> GAMASSNTAATNADSAWLEAQEEEEVGFPVRPQVPLRPMTYKAALDISHFLKEKGGLEGLIWSQRRQEILDLWIYHTQGYFPDWQNYTPGPGIRYPLTFGWCFKLVPVEPEKVEEANEGENNSLLHPMSLHGMEDAEKEVLVWRFDSKLAFHHMARELHPEY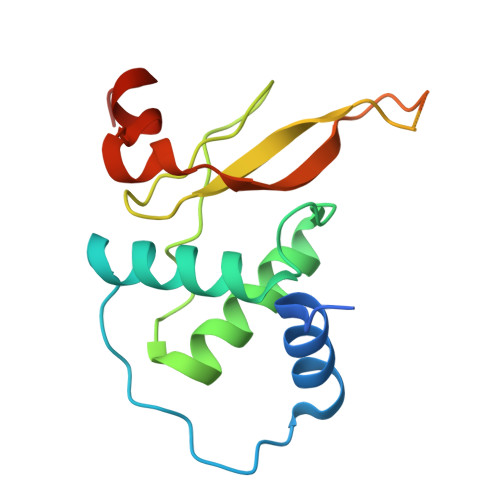YKDA>MKQYLELMQKVLDEGTQKNDRTGTGTLSIFGHQMRFNLQDGFPLVTTKRCHLRSIIHELLWFL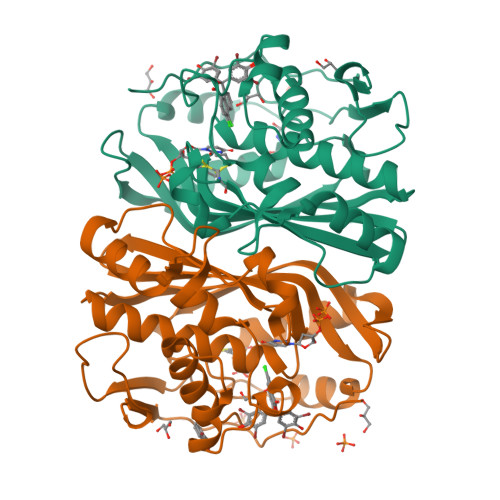QGDTNIAYLHENNVTIWDEWADENGDLGPVYGKQWRAWPTPDGRHIDQITTVLNQLKNDPDSRRIIVSAWNVGELDKMALAPCHAFFQFYVADGKLSCQLYQRSCDVFLGLPFNIASYALLVHMMAQQCDLEVGDFVWTGGDTHLYSNHMDQTHLQLSREPRPLPKLIIKRKPESIFDYRFEDFEIEGYDPHPGIKAPVAI[4x]>GERTEDYPKLLEYGLDKKVAGKLDEIYKTGKLAHAELDERALDALKEFPVDGALNVLGQFLESNLEHVSNKSAYLCGVMKTYRQKSRASQQGVAAPATVKGPDEDKIKKILERTGYTLDVTTGQRKYGGPPPHWEGNVPGNGCEVFCGKIPKDMYEDELIPLFENCGIIWDLRLMMDPMTGTNRGYAFVTFTN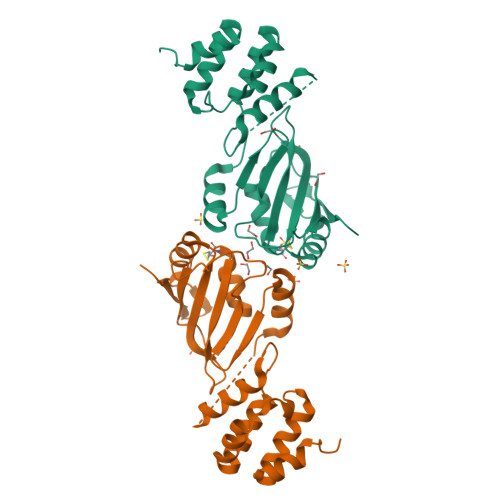REAAVNAVRQLDNHEIKPGKCLKINISVP[2x]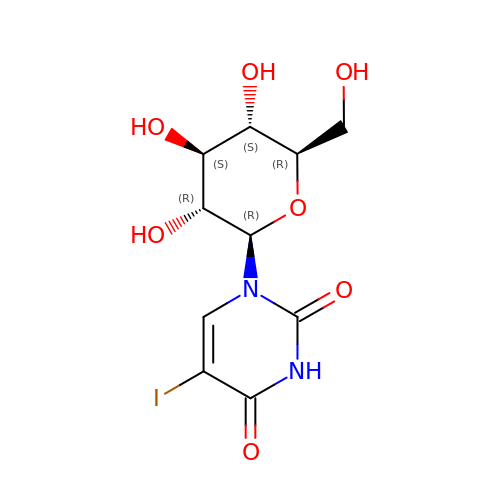1-(beta-D-glucopyranosyl)-5-iodopyrimidine-2,4(1H,3H)-dione | C10 H13 I N2 O7 | NKQVRMXGIOZKRJ-XSEHCYKFSA-N>MVYQVKDQEDFTKQLNEAGNKLVVIDFYATWCGPCKMIAPKLEELSQSMSDVVFLKVDVDECEDIAQDNQIACMPTFLFMKNGQKLDSLSGANYDKLLELVEKNK[2x]

Litopenaeus vannamei thioredoxin (LvTrx) is a redox protein with a molecular weight of 12 kDa, which catalyzes the reduction of the disulfide bond in different biological systems. The determination of the crystal structures of LvTrx under different redox conditions discloses a dimeric form mediated by a disulfide bond and other residues that are involved in the dimeric interface. The LvTrx contains four cysteines; two of them are engaged to form a catalytic disulfide bond (Cys32 and Cys35); Cys62 is not involved in any interactions, but in human thioredoxin (hTrx), it has been reported that Cys62 is readily S-nitrosylated, giving a SNO modification; and Cys73, which in previous studies, showed a dimeric behavior in the crystal system of hTrx and LvTrx, mediated by the interface disulfide bond through the Cys73 residue of each monomer. In an attempt to determine if the interface disulfide bond is viable to be reduced or if it is a consequence of a crystalline arrangement, we used X-rays as a tool to conduct experiments of radiation damage to monitor the reduction of the interface disulfide bond in two crystals of LvTrx.

During data collection, two crystal of LvTrx were diffracted at different transmissions, referred to below as LvTrx-1x (8% of transmission, 1.33 × 10 11 photons·s−1) and LvTrx-3x (27% of transmission, 4.14 × 1011 photons·s−1). In the case of the crystal of LvTrx-3x, the structure analysis showed that the catalytic disulfide bond was disrupted at a dose of 32 MGy. Despite the fact that cysteine mediated the interface disulfide bond, this residue exhibits a double conformation in the seven datasets. The disulfide bond was stable up to a dose of 85 MGy, in which the reduction was complete. The tolerance that the interface disulfide bond has to radiation damage is unusual, because this disulfide bond is exposed to the solvent with an ASA of ~50 Å2. This result suggests that the maintenance of this covalent interaction could depend on the residues involved in the dimer interface of the LvTrx. The analysis of our experiments with two crystals of LvTrx show a specific radiation damage in the catalytic and the interface disulfide bond as a result of the sequential increase in the absorbed dose during the collection of each dataset. This analysis shows that the catalytic disulfide bond deterioration is less tolerant to radiation damage than the disulfide bond located in the dimeric interface with a calculated absorbed dose of 32 MGy and 85 MGy, respectively. The disruption of the interface disulfide bond opens up the possibility that the dimeric form in LvTrx is also possible in solution.>MPNIKIFSGSSHQDLSQKIADRLGLELGKVVTKKFSNQETCVEIGESVRGEDVYIVQSGCGEINDNLMELLIMINACKIASASRVTAVIPCFPYARQDKKDKSRAPISAKLVANMLSVAGADHIITMDLHASQIQGFFDIPVDNLMAEPAVLKWIRENISEWRNCTIVSPDAGGAKRVTSIADRLNVDFALIHKERKKANEVDRMVLVGDVKDRVAILVDDMADTCGTICHAADKLLSAGATRVYAILTHGIFSGP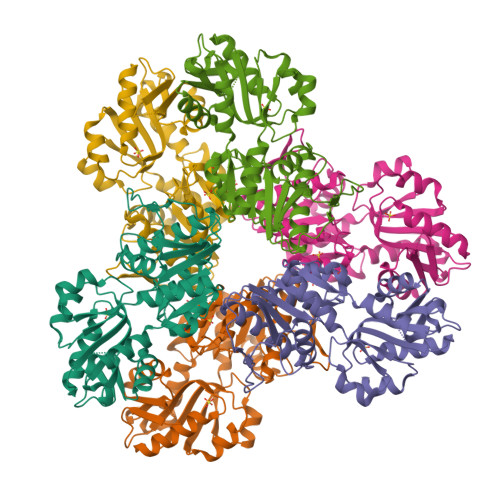AISRINNACFEAVVVTNTIPQEDKMKHCSKIQVIDISMILAEAIRRTHNGESVSYLFSHVPLLEHHHHHH[2x]>MAEAKVLSGAGLRGQVAGQTALSTVGQEGAGLTYRGYDVRDLAAAAIFEEVAYLLLYGELPNKQQLDAYLKKLQGQRDLPQALKEVLERIPKDAHPMDVMRTGASVLGTLEPELSFDQQRDVADRLLAAFPAIMTYWYRFTHEGQRIDCNSDEPTIGGHFLALLHGKKPSELHVKVMNVSLILYAEHEFNASTFTARVCASTLSDLYSCVTGAIGSLRGPLHGGANEAA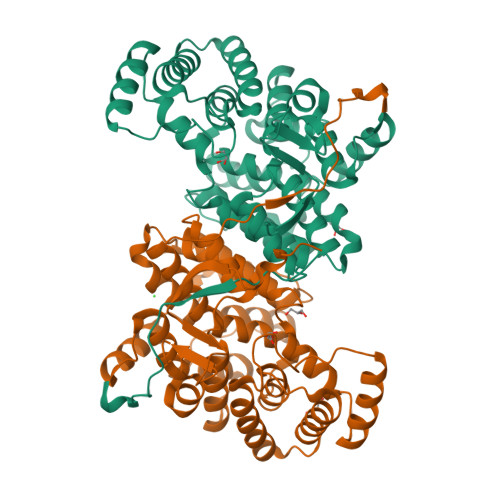MELIERFSSPQEATAELLKMLERKDKIMGFGHAIYKDSDPRNEVIKGWSKQLADEVGDKVLFAVSEAIDKTMWEQKKLFPNADFYHASAYHFMGIPTKLFTPIFVCSRTSGWTAHVFEQRANNRIIRPSAEYTGVEQRAFVPLEQR[2x]>[4x]GHVSDLPRISVAAPR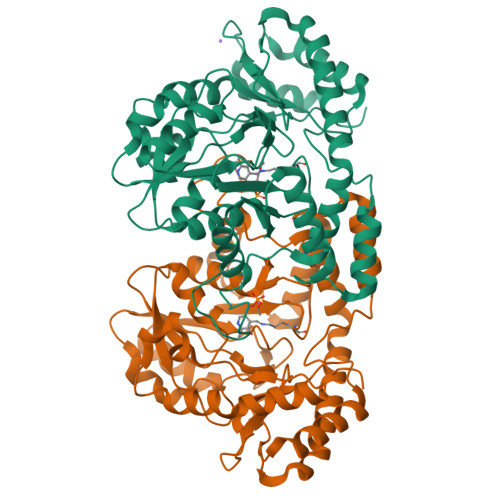LDGNERDYVLECMDTTWISSVGRFIVEFEKAFADYCGVKHAIACNNGTTALHLALVAMGIGPGDEVIVPSLTYIASANSVTYCGATPVLVDNDPRTFNLDAAKLEALITPRTKAIMPVHLYGQICDMDPILEVARRHNLLVIEDAAEAVGATYRGKKSGSLGDCATFSFFGNKIITTGEGGMITTNDDDLAAKMRLLRGQGMDPNRRYWFPIVGFNYRMTNIQAAIGLAQLERVDEHLAARERVVGWYEQKLARLGNRVTKPHVALTGRHVFWMYTVRLGEGLSTTRDQVIKDLDALGIESRPVFHPMHIMPPYAHLATDDLKIAEACGVDGLNLPTHAGLTEADIDRVIAALDQVLV Strikingly, the SidE- and MavC-type enzymes, two recently identified effector families from the bacterial pathogen Legionella pneumophila, can ubiquitinate host substrates through non-canonical mechanisms without engaging any of the conventional ubiquitination machinery. The genomic cluster of MavC encodes three effector proteins: Lpg2147 (MavC itself), Lpg2148 (MavC paralog A, or MvcA), and Lpg2149. Taken together, our data show that MavC can catalyze deamidation, ubiquitination, and deubiquitination by using the same active pocket. In addition to MavC and MvcA, the same genomic cluster in L. pneumophila also encodes a small effector protein, Lpg2149, which has been shown to interact with both enzymes and inhibit their deamidation activities.

The inhibitory role of Lpg2149 in the MavC system is reminiscent of the function of SidJ in the SidE system, although their operation mechanisms are distinct from each other. To understand the detailed molecular mechanisms of Lpg2149-mediated inhibition, we determined the crystal structures of MavC–Lpg2149 and MvcA–Lpg2149 complexes (X-ray statistics in Table 1). The asymmetric unit contains one Lpg2149 and one enzyme for both structures, highlighting a 1:1 molar ratio of the complex formation. Both structures adopt a similar assembly, with the Lpg2149 monomer binding to the connecting region between Catalytic and HBD domains. Lpg2149 forms similar and extensive hydrogen bonding and hydrophobic interactions with MavC and MvcA, which are mainly mediated by the N-terminal α-helix (aa 11–37) and a helix-loop motif (aa 74–86) of Lpg2149. Structural superimposition of MavC in Ub- and Lpg2149-bound states shows that Lpg2149 and Ub occupy a similar binding position and form severe steric clashes with each other, indicating that Lpg2149 can interfere with the interactions between Ub and MavC/MvcA. Upon binding to the enzymes, this C-terminal α-helix folds back and occupies the groove of the very same Lpg2149 molecule. The Catalytic–HBD dual domain of MavC adopts a similar conformation with or without Lpg2149. Given that MavC has the pre-formed Lpg2149 binding surface, we anticipated that MavC may have a stronger binding affinity to Lpg2149 than MvcA. Isothermal titration calorimetry (ITC) experiments confirm that the binding of Lpg2149–MavC (~0.57 nM) is ~50-fold stronger than that of Lpg2149–MvcA (~28.08 nM). Further SEC experiments show that the V20D/L23D/L24D mutant cannot form a stable complex with MavC like WT Lpg2149.

> SGTFFKDYQKKNVMRLLQDSLEKIINEWLKTDDESHTKLKSLQELSEMDINATSFAEHSPLPDFVTRLWLDPHKALDAMDKNISKNEIRKLIKETAREIELVFTH;> SMTTSKLEKTGLHVHEKIKHMVKNYGTMITGIPAEILGQNEAEISVGYVKKMGNMKENIAEVVRKSEMTQPTNSCGKASNEVCDLLLGTEGASEFEKSSYQVLSGDGSNLKGSLPNKNLLVRVEMDRFNAPQKYQKIKREEFNPETAEKNKIYLLEDQLVYLDIFGKVIDLGQTSDTCHRLFNAITTPFYQNYILYDEYIDPEESAEEAAMFEMGEIVKAKMKNIDCWTATHSFTIFVPESDSEDTRTLYPYQAYWTSHTLQQWFSGDKDEKLSRLGIDGYIEKLALLGTTTDSKIRSSIYGELFSPPGKEHVFCTGMNEKFSPLRVKFKVTEVNPEIALQNLEEVQEFIDTNYPGENAKDQCELYKIKAQEAMTKQLEMRLLIEP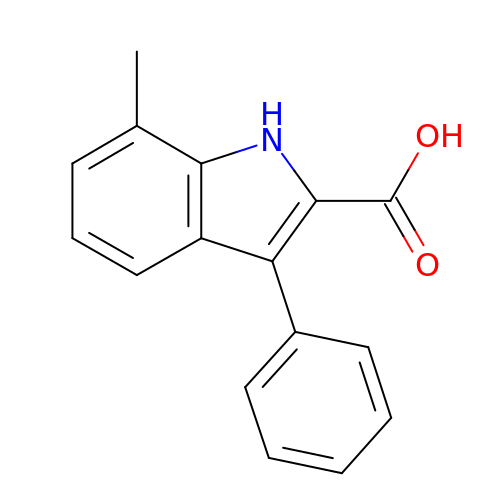7-methyl-3-phenyl-1H-indole-2-carboxylic acid | C16 H13 N O2 | OSOLISRTJWBBIW-UHFFFAOYSA-N>GPMEEKALIGIEDFLKVDLRVAKVLSAERVEGSEKLLKLTLSLGDEERTVVAGIAKYYTPEELVGKKIVIVANLKPRKIFGIESQ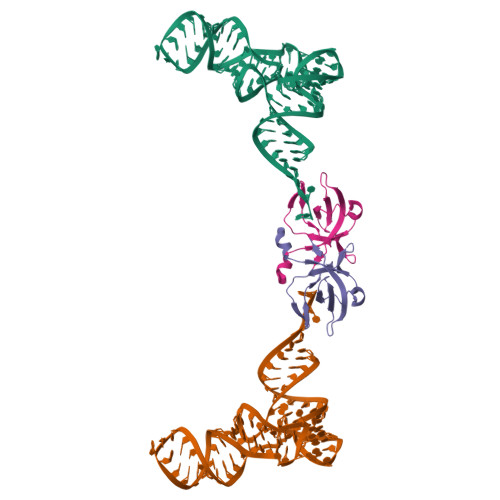GMILAASDGENLSVIVPDRDVKEGAKLS[2x]> PKYTKSVLKKGDKTNF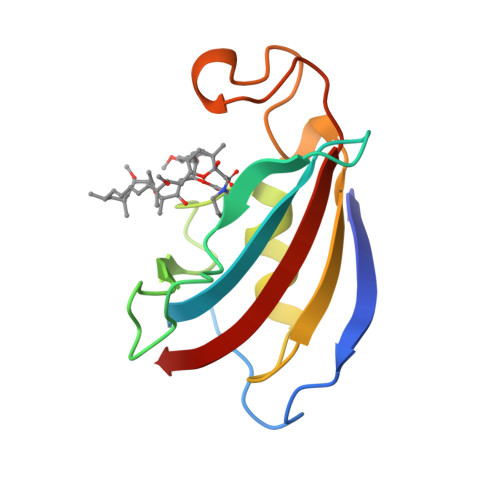PKKGDVVHCWYTGTLQDGTVFDTNIQTSAKKKKNAKPLSFKVGVGKVIRGWDEALLTMSKGEKARLEIEPEWAYGKKGQPDAKIPPNAKLTFEVELVDID> M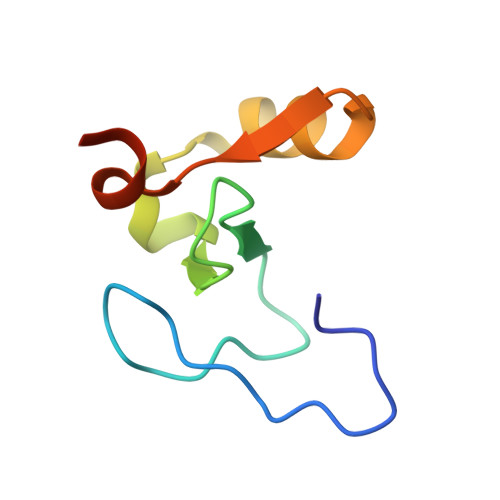GHSSSDPVYPCGICTNEVNDDQDAILCEASCQKFFHRICTGMTETAYGLLTAEASAVWGCDTCMADKDVQ>[6x]SVDREEMIERFANFLREYTDEDGNPVYRGKITDLLTITPKRSVAIDWMHLNSFDSELAHEVIENPEEGISAAEDAIQIVLREDFQREDVGKIHARFYNLPETLMVKDIGAEHINKLIQVEGIVTRVGEIKPFVSVAVFVCKDCGHEMIVPQKPYESLEKVKKCEQCGSKNIELDVNKSSFVNFQSFRIQDRPETLKGGEMPRFIDGILLDDIVDVALPGDRVIVTGILRVVLEKREKTPIFR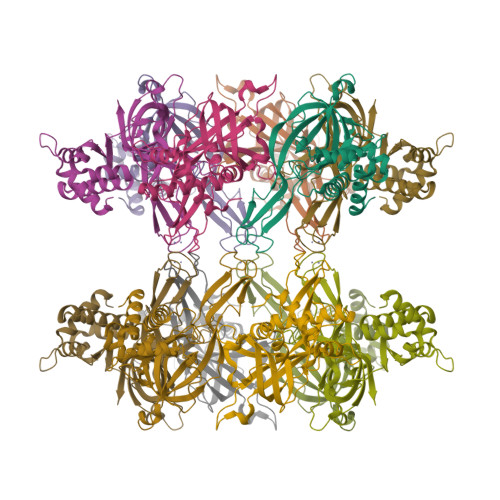KILEVNHIEPVSKEI> MDNWESITKSYYTGFAISKTVESKDKDGKPVRKEVITQADLTTACNDAKASAQNVF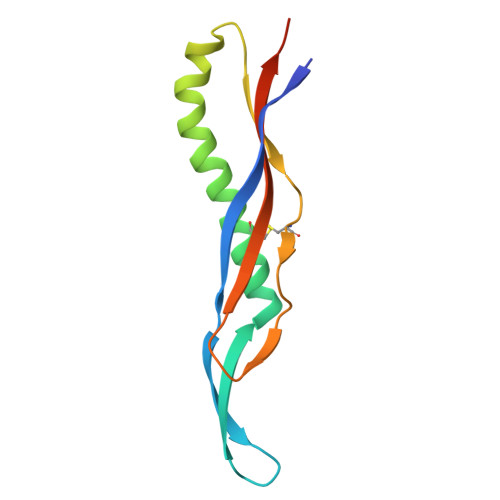NQIKLTLSGTWPNSQFRLVTGDTCVYNGSPGEKTESWSIRAQVEGDIQRSVPDHHHHHH>[2x]CRQKGAGSAGTGSETNSQEVRSQMRSTCLIIPKERFRTMAKEISKKEGHDVHIAEAALDMLQVIVESCTVRLLEKALVITYSGKRTRVTSKDIETAFMLEHGPLLE;>[2x]LADHVSVGETQIPKASTQHLLRKAGSLSAAGDTEVPIRGFVHMKLHKLVQKSLLAMQLAKRKTIMKSDVKKAAELMHLPVFAIPTKDSGAKGSV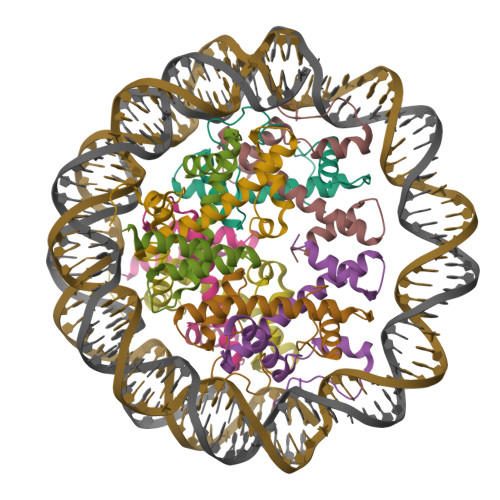FLS;>ESKEGSRSSKAKLQISVARSERLLREHGGCSRVSEGAAVALAAAIEYFMGEVLELAGNAARDSKKVRISVKHITLAIQNDAALFAVVGKGVFSGAGVSLISVPIPRKKARKTTEKEASSPKKKAAPKKKKAASKQKKSLSDKELAKLTKKELAKYEKEQGMSPGY[2x];>[2x]MATQKETTRKRDKSVNFRLGLRNMLAQIHPDISVQTEALSELSNIAVFLGKKISHGAVTLLPEGTKTIKSSAVLLAAGDLYGKDLGRHAVGEMTKAVTRYGSAK> KRRQTSMTDYY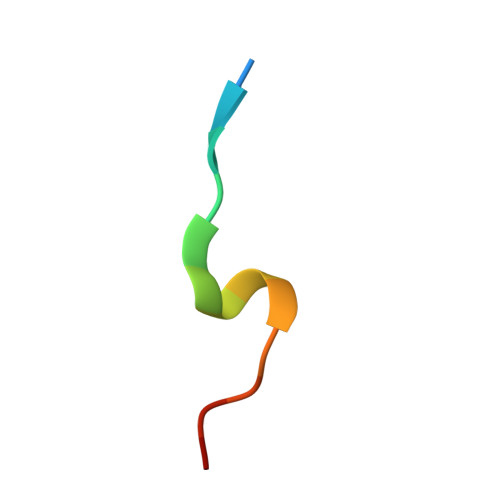HSKR> NNPYLFRSNKFLTLFKNQHGSLRLLQRFNEDTEKLENLRDYRVLEYCSKPNTLLLPHHSDSDLLVLVLEGQAILVLVNPDGRDTYKLDQGDAIKIQAGTPFYLINPDNNQNLRILKFAITFRRPGTVEDFFLSSTKRLPSYLSAFSKNFLEASYDSPYDEIEQTLLQEEQEGVIVKMP;> DKPFNLRSRDPIYSNNYGKLYEITPEKNSQLRDLDILLNCLQMNEGA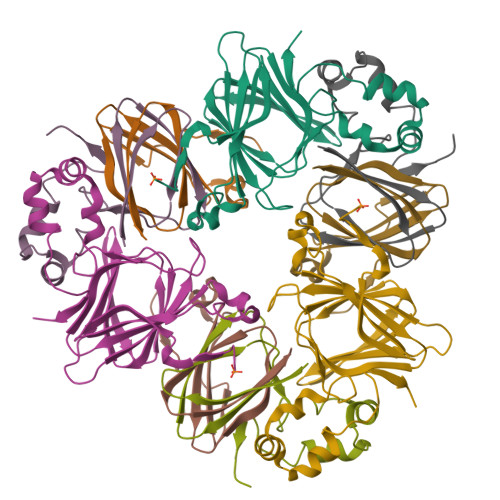LFVPHYNSRATVILVANEGRAEVELVGLEQQQ;> MQLRRYAATLSEGDIIVIPSSFPVALKAASDLNMVGIGVNAENNERNFLAGHKENVIRQIPRQVSDLTFPGSGEEVEELLENQKESYFVDGQP>[2x]HNHNHNHNHNHNAA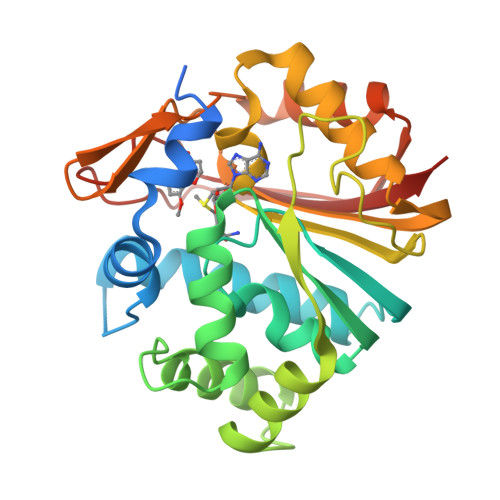AENLYFQSGFTSKDTYLSHFNPRDYLEKYYKFGSRHSAESQILKHLLKNLFKIFCLDGVKGDLLIDIGSGPTIYQLLSACESFKEIVVTDYSDQNLQELEKWLKAAPAAFDWSPVVTYVCDLEGNRVKGPEKEEKLRQAVKQVLKCDVTQSQPLGAVPLPPADCVLSTLCLDAACPDLPTYCRALRNLGSLLKPGGFLVIMDALKSSYYMIGEQKFSSLPLGREAVEAAVKEAGYTIEWFEVISQSYSSTMANNEGLFSLVARKLS>[12x]MVMAVAANKRSVMTLYSGKDDLKSHQVRLVLAEKGVGVE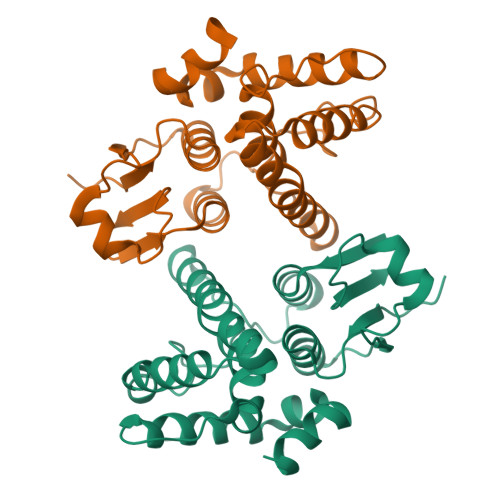ITYVTDESTPEDLLQLNPYPEAKPTLVDRELVLYNAQIIMEYLDERFPHPPLMPVYPVARGTSRLMMYRIERDWYSLAEKIQKNDAQARQELKEGILSLAPIFADTPYFMSEEFSLVDCYLAPLLWRLPAYGIDLEGQGAKEIKQYMVRLFERKTFQDSLTEEEKELARNAENLYFQSHHHHHHWSHPQFEK> GSKMSDVKCTSVVLLSVLQQLRVESSSKLWAQCVQLHNDILLAKDT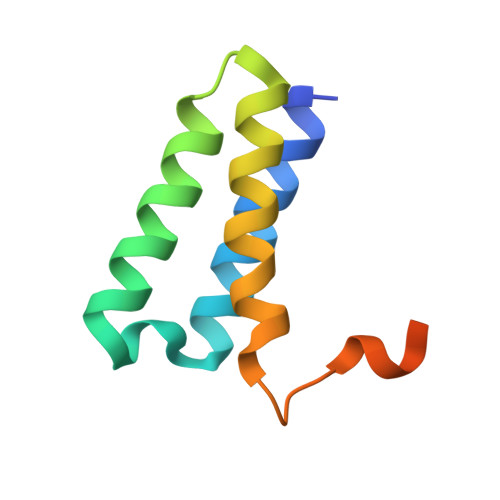TEAFEKMVSLLSVLLSMQGAVDINRLCEEMLDNRATLQ>[2x]MEEPEEPADSGQSLVPVYIYSPEYVSMCDSLAKIPKRASMVHSLIEAYALHKQMRIVKPKVASMEEMATFHTDAYLQHLQKVSQEGDDDHLDSIEYGLGYDCPATEGIFDYAAAIG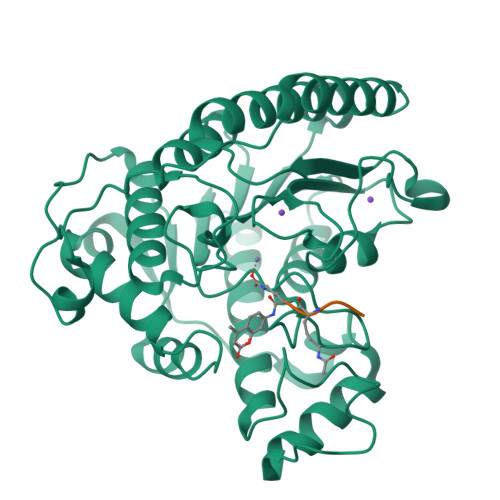GATITAAQCLIDGMCKVAINWSGGWHHAKKDEASGFCYLNDAVLGILRLRRKFERILYVDLDLHHGDGVEDAFSFTSKVMTVSLHKFSPGFFPGTGDVSDVGLGKGRYYSVNVPIQDGIQDEKYYQICESVLKEVYQAFNPKAVVLQLGADTIAGDPMCSFNMTPVGIGKCLKYILQWQLATLILGGGGFNLANTARCWTYLTGVILGKTLSSEIPDHEFFTAYGPDYVLEITPSCRPDRNEPHRIQQILNYIKGNLKHVVIEGRGSHHHHHH> A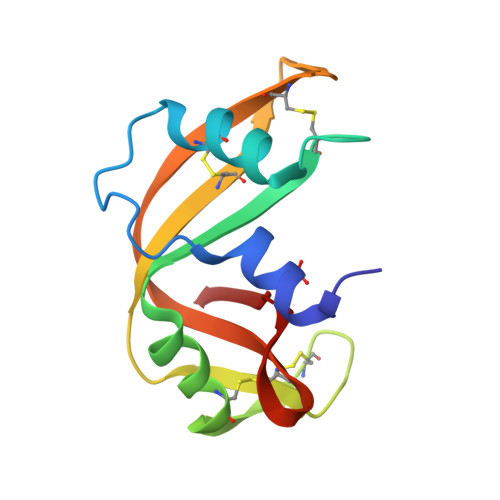ESSADKFKRQHMDTEGPSKSSPTYCNQMMKRQGMTKGSCKPVNTFVHEPLEDVQAICSQGQVTCKNGRNNCHKSSSTLRITDCRLKGSSKYPNCDYTTTDSQKHIIIACDGNPYVPVHFDASV Diperodon | C22 H27 N3 O4 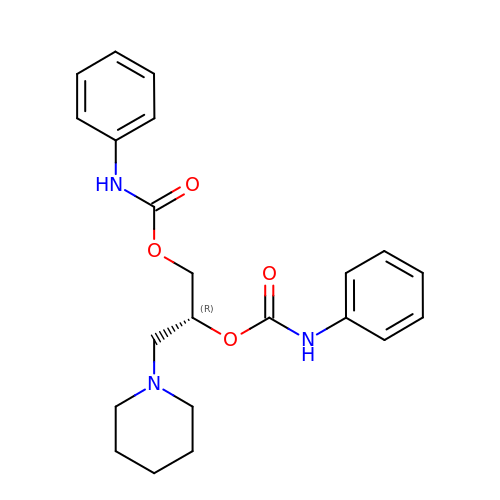| YUGZHQHSNYIFLG-HXUWFJFHSA-N RtGH124 is the defining member of CAZY family GH124. Unusually for R. thermocellum, RtGH124A is not targeted to the multi-enzyme cellulosome complex of the organism but instead consists of a ‘dockerin’ domain which instead targets the enzyme to the cell surface of the bacterium, followed by a CAZY GH124 catalytic domain; RtGh124 is therefore an unusual enzyme if its primary role is in cellulose degradation yet it is not part of the cellulose complex. Here, we show that the metal-ion site of GH124 can accommodate a variety of metal ions (but not Ca2+) and that the histidine is modified by a carbonyl group at C2 to make 2-oxohistidine (but only at a fraction of approximately 0.5). Metal binding also occurs with a stoichiometry of approximately 0.5 (in solution by ITC and in the crystal through occupancy refinement) and we are thus unable to deconvolute whether the 2-oxohistidine is required for metal binding or antithetical to it.

In passing, we determined a series of structures of GH124 co-crystallized with cellohexaose which revealed the unusual binding of a contaminant, a terminally fructosylated cellooligosaccharide, with unambiguous density at ∼1 Å resolution. Clear electron density indicated that the reducing-end sugar was not glucose, as expected, but a 1–4-linked fructose moiety. The hexasaccharide appears not to be cleaved, as four to six molecules of each chain have been observed in all of the structures (data not shown). Enzyme subsites −4 to −1 are occupied by one molecule and +1 to +4 by another, with both of them stabilized in the crystal by a second molecule in the same asymmetric unit. Our initial thought was that the fructosylated oligosaccharide would be likely to represent a very minor contaminant in the G6 preparation, one somehow selected by the enzyme owing to tighter binding and/or inhibitory potential. The originally purchased G6 sample contained an approximately 1:1 ratio of G6 and G5F (but subsequently purchased batches were 100% G6), highlighting that the unusual observed species was simply a contaminant in the commercial supply of G6 available at that time. Manganese is coordinated by Asp141, Gln172, Glu175, His176, His264 and a water molecule. High-resolution structures of RtGH124 (1.40–0.94 Å) have revealed an unambiguous modification of C2 of His264. In the case of manganese, the metal and the His264 modification both display partial occupancies of 0.7 and 0.3, respectively.

>[2x]GPAPANTQSGILNDGYFPPGTSKHELIARASSLKVSEVKAIIKKQVDEHWDVIRDVCGFKNKEVAYAFFFGMATRESTFRAATETGSGASHAFGPLQTAETAYANANPNYMPEHNVPEMHQYDFTEYNFYDVGISVHMGIRHFLHFARLAKEKYSGRDIARHGLMGYNTGWIDGADESWIVRYADETAALGAWYLRNNHMSDDEFTWDTDPRVDRSNPWEIYY>[2x]GSHMRGREEKAPEEPQPVKMPENNSVVAATWNAVQLEDSLGMEVGYRLIPMVDFQQDGELLGRIRSIRKKFAQDMGFLPPVVHIRDNMDLQPARYRILMKGVEIGSGDAYPGRWLAINPGTAAGTLPGEKTVDPAFGLDAIWIESALKEQAQIQGFTVVEASTVVATHLNHLIGQF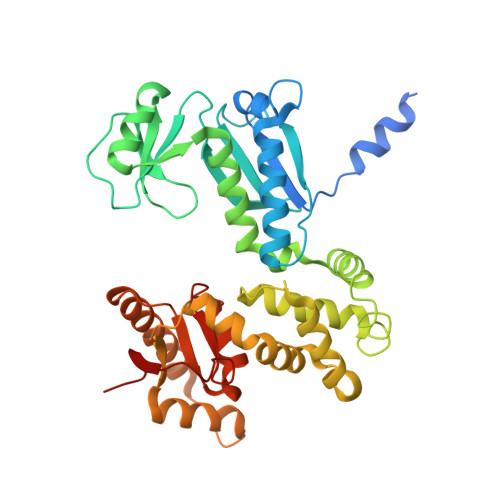SAELFGRQEAQQLLDRVSQEMPKLTEDLVPGVVTLTTLHKVLQNLLAEKVPIRDMRTILETLAEHAPLQSDPHELTAVVRVALGRAITQQWFPGNEEVQVIGLDTALERLLLQALQGGGGLEPGLADRLLAQTQEALSRQEMLGAPPVLLVNHALRPLLSRFLRRSLPQLVVLSNLELSDNRHIRMTATIGGK> LICVNENGGCEQYCSDHTGTKRSC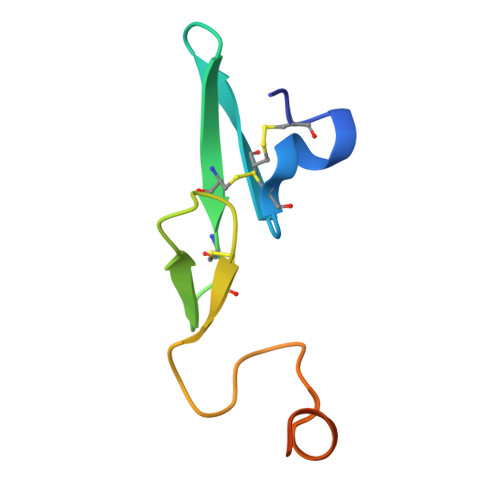RCHEGYSLLADGVSCTPTVEYPCGKIPILEKRNASKPQGR>MTGHIDPTKEVFAQFRANDREGPIHMLNLVRLRPRAAYPDGRETTGAEAYAAYGRDSGPVFERLGGKVVWQGQFELMLIGPQDEHWDHVFIAEYPSVA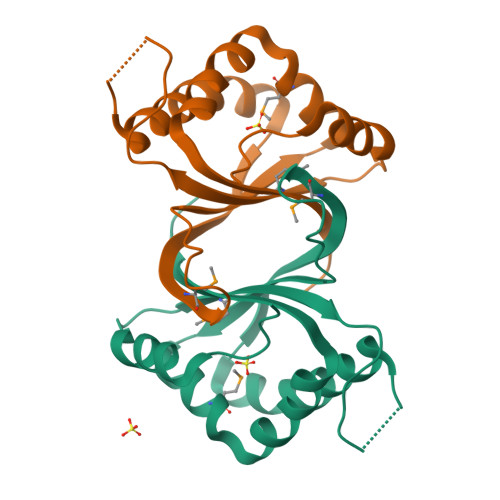AFVEMIRDPVYREAVKHRQAAVEDSRLIRLKPLKPGKGFGEIPT[4x]In the present work, we present the purification and biochemical characterization of a mJRL from the stem of Ananas comosus (AcmJRL). Size-exclusion chromatography clearly showed that AcmJRL is a homodimeric lectin in solution. AcmJRL adopt the expected β-prism fold with the three characteristic Greek key four-stranded β-sheets (β1–2 + β11–12, β3–6 and β7–10) and all the connecting loops well defined in the electron density. The structure of AcmJRL is the second structure of a mJRL reported with two carbohydrate-binding sites per monomer after BanLec.

Two structures of AcmJRL in complex with D-mannose (AcmJRL:Man) and methyl-α-D-mannopyranoside (AcmJRL:MeαMan) were obtained at 2.75 Å and 1.9 Å respectively. These structures belong to the P6422 space group but with significantly different c axes (257.3 Å and 204.4 Å respectively) indicating different packing. In both cases, the asymmetric unit contains two molecules. They form the side-by-side dimer in AcmJRL:Man and the tail-to-tail dimer in AcmJRL:MeαMan. The overall structures of the AcmJRL:Man and AcmJRL:MeαMan complexes are similar to the AcmJrl structure, with rms deviation between carbon α of the four monomers of 0.75 Å and 0.7 Å respectively. In the AcmJRL:MeαMan complex, a methyl-α-D-mannopyranoside molecule was modeled in each of the two binding-sites 1. The interactions with AcmJRL were all conserved except the hydrogen bond between O5 and the hydroxyl group of Ser133, which rotated 120° as a result of steric hindrance with the methyl group of this ligand. For the binding site 2, a methyl-α-D-mannopyranoside molecule was only modeled in monomer A. The hydrogen bonds between the ligands and the protein in the AcmJRL:Man complex where conserved in the AcmJRL:MeαMan complex, despite a slight rotation of the ligand potentially due to the close proximity of the ligand methyl and the side chain of His36. An extra density is also present in the binding site 2 of monomer B but the quality was not sufficient to properly fit the ligand. This is likely a consequence of an insufficient occupation of this site due to a steric hindrance with the methyl-α-D-mannopyranoside bound in the binding site 1 of a symmetric molecule in the crystal.

>[2x]SGLVKLGLWGGNEGTLQDIDGHPTRLTKIVIRSAHAIDALQFDYVEDGKTFAAGQWGGNGGKSDTIEFQPGEYLIAIKGTTGALGAVTNLVRSLTFISNMRTYGPFGLEHGTPFSVPVASGRIVAFYGRFGSLVDAFGIYLMPY> GQIRYSVPEETEKGYIVGNISKDLGLEPRELAERGVRIISKGKTQLFSLSPRSGSLVTAGRIDREELCAQSATCLLNFKVLVEDRVKLYGVEVEVVDINDNAPKFEAENLFVKISEIAAPGARYPLPEAVDPDVGINSLQSYQLSPNRHFSLHLQTGDDGTINPELVLERTLDREEEPTHHLVLTAYDGGNPRRSSTALIQVTVLDTNDNAPVFDQPVYRVKVLENVAPGTLLLTVRASDPDEGANGKVTYKFRKI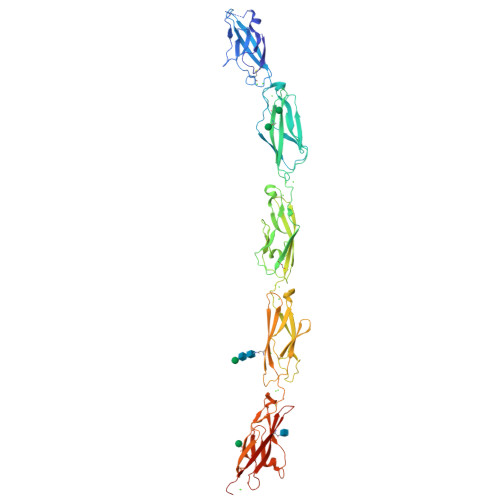NEKHSLLFHLHENTGEMTVAKNLDYEECSLYEMEIQAEDGGGLKGRTKVVVMVEDVNDNRPEVTITSLFSPVREDAPPGTVILLFNAHDQDSGKNGQVVCSIQENPSFKLENSVDDYYRLLTAQILDREKASEYNITVTATDRGTPSMSTEVHITLYVADINDNPPAFSQTSYSVYLPENNPRGTSIFSVSAHDPDDEENAKVTYSLVENTIQGAPLSSYVSINSDTGVLYALQSFDYEQFQNLQMQVKASDNGHPPLSSNVSLSVFLLDQNDHHHHHHHH> ALTRNLHPIGKIAITSVHLKLPILKGLSNDNLSAGAGTMKADQKMGEGNYALAGHYMTNQGILF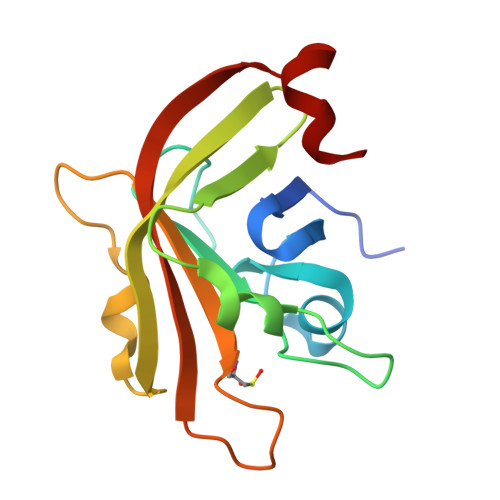SPLKNVQTGDTVAITNMKKVYTYKVTTKQIVNETQVQWIDDVAGKKLITLVTCASPTEGEVDRIIVQGELQSVKKANQKNLKIFL> MPSIRVVNLKKYFGKVKAVDGVSFEVKDGEFVALLGPSGCGKTTTLLMLAGIYKPT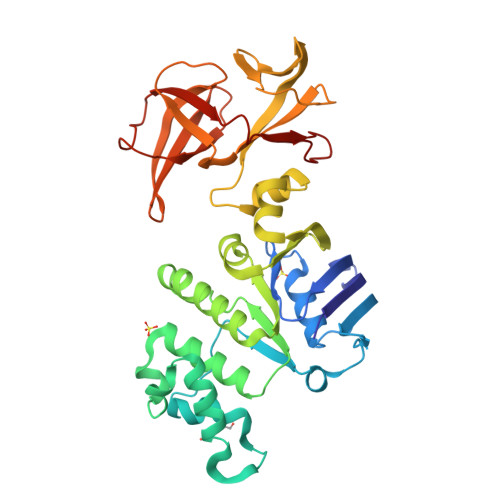SGEIYFDDVLVNDIPPKYREVGMVFQNYALYPHMTVFENIAFPLRARRISKDEVEKRVVEIARKLLIDNLLDRKPTQLSGGQQQRVALARALVKQPKVLLFDEPLSNLDANLRMIMRAEIKHLQQELGITSVYVTHDQAEAMTMASRIAVFNQGKLVQYGTPDEVYDSPKNMFVASFIGNPPTNFLRDFSVSVENKQTILKRDDVIIKLPEPVDVKLKEVVVGIRPEHCRISRERVENSIPGVVYVVEPLGRDIIVNVKTEKGEIIKVFGDTGKAPQPGENVFLVPDLRKIHLFNPETEETIL> YEEKEESNLAATKSMVKIAEQYSKRIEEEK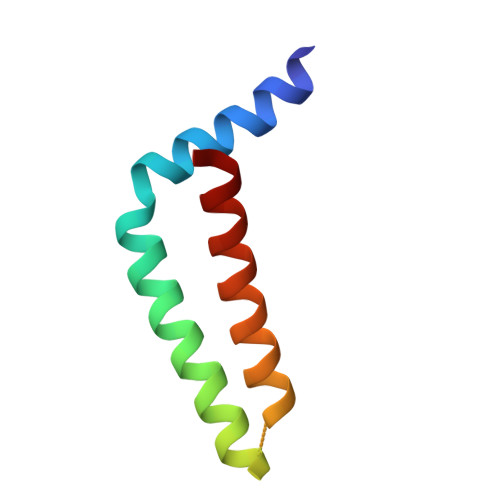ELTEEELKTRYVGRQDPKKHLSETADETLENNIVSVLTA> SRMQEKHMRIRVKLLDSTVELFDIEPKCDGQVLLTQVWKHLNLIECDYFGLEFKNVQSYWIWLEPMKPIIRQVRKPKNAVLRLAVKFFPPDPGQLQEEYTRYLFALQLKRDLLEERLTCTANTAALLISHLLQSEIGDYDETLDREHLKANEYLPNQEKSLEKILDFHQRHTGQTPAESDFQVLEIARKLEMYGIRFHMASDREGTKINLAVSHMGVLVFQGTTKINTFNWSKVRKLSFKRKRFLIKLHPEVHGPYQDTLEFLLGSRDECKNFWKICVEYHTFFRLSD

FARP1 (FERM, RhoGEF and pleckstrin domain-containing protein 1) and its close homolog FARP2 were identified as guanine nucleotide exchange factors (GEFs) for RhoGTPases that play regulatory roles in neuronal development. FARP1 and FARP2 share a conserved domain architecture, containing a N-terminal 4.1, ezrin, radixin and moesin (FERM) domain, which is followed by a long linker (~200 residues) that connects to a Dbl-homology (DH) domain and two pleckstrin homology (PH) domains. We determined crystal structures of the FERM domains of zebrafish FARP1 (zfFARP1), mouse FARP2 (mFARP2) and zebrafish FARP2 (zfFARP2). As expected from their high degree of sequence identity (>60%), the structures of these FERM domains are very similar to one another, with root mean square deviations within 1.0 Å.

FARP2 also interacts with PlexinA family members, contributing to both Plexin-mediated repulsive axon guidance and dendritic development. The corresponding site in the FERM domains of FARP1 and FARP2 contains a negatively charged residue (Asp97, Glu100 and Asp107 in zfFARP1, mFARP2 and zfFARP2, respectively), suggesting that it cannot serve as a phosphatidylinositol binding site in these FERM domains. In particular, the FERM domains of FARP1 and FARP2 contain a Lys-Arg-Lys-Arg (KRKR) motif in the loop connecting strands β5 to β6 in the F3 subdomain, which is highly conserved in FARP1/2 from different species. Overall, the surface of these FERM domains show highly polarized surface electrostatic potential, with one side positively charged while the opposite side negatively charged. Interestingly, both the FERM domains of mFARP2 and zfFARP2 form similar head-to-tail packing patterns in the crystal lattices, as a result of interactions between the positively charged and the negatively charged faces of the proteins. These packing patterns lead to a linear array of the FERM molecules, which may cause the oligomerization and precipitation of the proteins. The first arginine residue in the KRKR motif (Arg277) in the FERM domain of mFARP2 makes a salt bridge with Asp216 from the neighboring protomer in the linear array. The linear packing of the FERM domains of mFARP2 and zfFARP2 in our crystal structures suggest a potential mechanism for the oligomerization of these FERM domains. The KRKR motif in the FERM domains responsible for phospholipid binding is buried in the oligomerization interface. We speculate that the oligomerization, if occurs in the cell, could be a mechanism for regulating membrane targeting of FARP1 and FARP2.(2R,4R)-N~1~-(4-CHLOROPHENYL)-N~2~-[3-FLUORO-2'-(METHYLSULFONYL)BIPHENYL-4-YL]-4-METHOXYPYRROLIDINE-1,2-DICARBOXAMIDE | C26 H25 Cl F N3 O5 S | 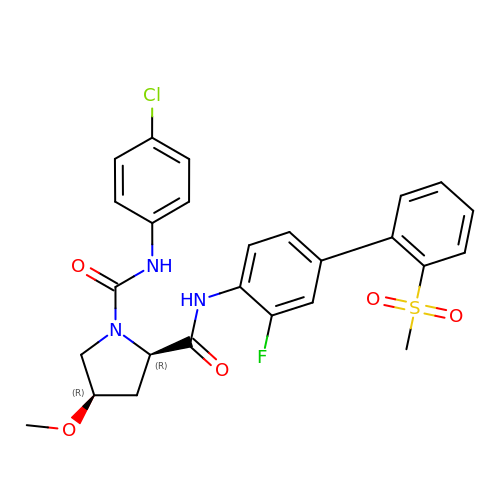QBTQRXKLWHEJQY-AUSIDOKSSA-N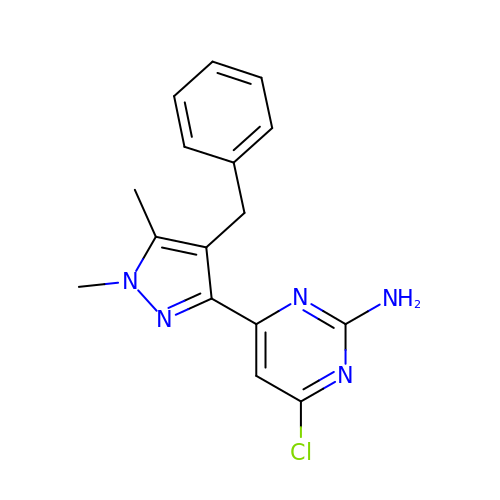4-chloranyl-6-[1,5-dimethyl-4-(phenylmethyl)pyrazol-3-yl]pyrimidin-2-amine | C16 H16 Cl N5 | VSMTYSWGHKYXOF-UHFFFAOYSA-N>MLEVIATCLEDVKRIERAGGKRIELISSYTEGGLTPSYAFIKKAVEAVQIPIHVMIRPHAKSFTYTEEEIEMMKEDIVVAQKLGVAGVVLGVLNERNEVAEEKLADLLSVVDGINVTYHRAIDDIENPVEAM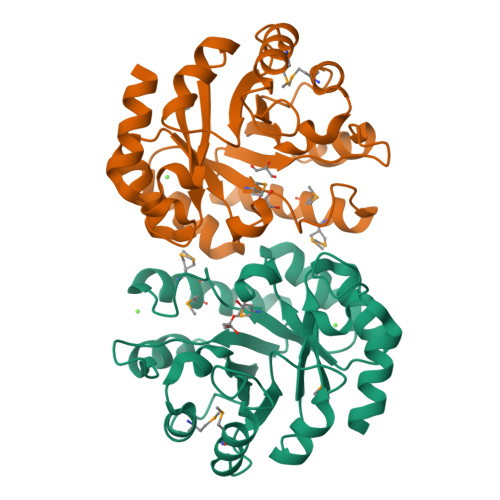RTLKKFHKVTHVLTSGGQGNIVDNIPVLTDMQKISDGQIQLVVGAGVTKENIKQLLNETGISQAHVGTAVREGKSCFAEIDLNLVQELVQIIQAGENLYFQ[2x]>MGNIILDLLLLLLTIIYSYLEALVKVFFPRKRKSVAGEIVLITGAGHGIGRWTAYEFAKQKSRLVLWDINKHGVEETAAECRKLGATVHTFVVDCGNREDIYNSVKQVKKEVGDVTILVNNAGTVYPADLLSTKDEEITKTFEINILGHFWITKALLPSMIKRNHGHIVTVASVCGHGVIPYLIPYCSSKFAAVGFHRALTLELQTLGITGIKTSCLCPVFVNTGFTKNPSTRLWPILETDTVARSLIDGILTNKKMIFVPSYYNIYLILDKFLPERALAAINHLQNIQFEAVIGHKTRMKGSGHHHHHHHHHHH[2x]

Hydroxysteroid 17-beta-dehydrogenase 13 (HSD17B13) is a hepatic lipid droplet-associated enzyme that is upregulated in patients with non-alcoholic fatty liver disease. Recently, there have been several reports that predicted loss of function variants in HSD17B13 protect against the progression of steatosis to non-alcoholic steatohepatitis with fibrosis and hepatocellular carcinoma. Here we report crystal structures of full length HSD17B13 in complex with its NAD+ cofactor, and with lipid/detergent molecules and small molecule inhibitors from two distinct series in the ligand binding pocket. The overall structure of each HSD17B13 subunit could be divided into two parts: (i) the catalytic core domain (residues 29–259) that contained the cofactor binding site and the catalytic center and (ii) the membrane anchoring domain that consisted of the N-terminal helix (N2-P28) which was highly hydrophobic and a C-terminal proximal helix-turn-helix motif (P260-N286) which formed an amphipathic patch on the protein surface.

We could remove compound 1 from these crystals by soaking with buffer containing NAD+ only and obtained NAD+ bound dog HSD17B13 crystals (apo Dog WT or apo hereafter). The nicotinamide nucleotide of NAD+ interacts with the putative catalytic triad of HSD17B13 (S172, Y185, and K189)23 and a long loop in HSD17B13, loop P218-T239. The adenine nucleotide of NAD+ forms hydrogen bonds with side chain of D67 and D93, and the main chain of C94. A prominent feature of the apo HSD17B13 structure is that the putative substrate-binding site is completely blocked by the C-terminal peptide beyond the helix-turn-helix motif. This peptide, N286-K300 (C terminus), interacted extensively with the long loop P218-T239. When a steroid molecule was docked in the active sites of the apo dog and human HSD17B13 by homology modeling, the molecule would clash with the C-terminal peptide and loop P218-239. In fact, repeated soaking with substrate β-estradiol failed to result in ligand binding. First, filling the pocket with the C-terminal peptide stabilizes HSD17B13. Second, access to the substrate site needs to compete with the C-terminal peptide, which may reduce the catalytic efficiency of HSD17B13 with any substrate. The apo HSD17B13 has essentially the same structure in different crystals, thus it may closely resemble the protein on the surface of the lipid-droplet in the absence of inhibitors.> EIKREYKEMEGSPEIKSKRRQFHQ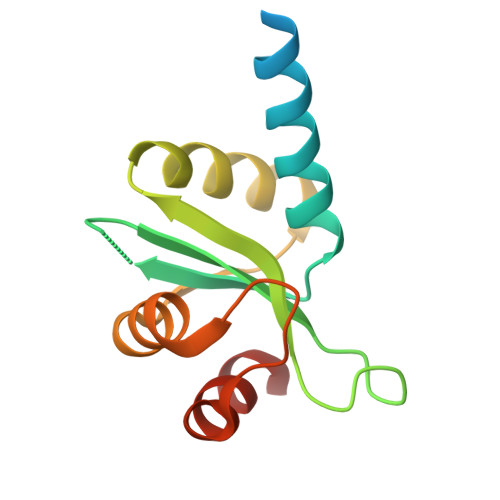EIQSRNMRENVKRSSVVVANPTHIAIGILYKRGETPLPLVTFKYTDAQVQTVRKIAEEEGVPILQRIPLARALYWDALVDHYIPAEQIEATAEVLRWLE> SYSGPIVVDPVTRIEGHLRIEVEVENGKVKNAYSSSTLFRGLEIILKGRDPRDAQHFTQRTCGVCTYTHALASTRCVDNAVGVHIPKNATYIRNLVLGAQYLHDHIVHFYHLHALDFVDVTAALKADPAKAAKVASSISPRKTTAADLKAVQDKLKTFVESGQLGPFTNAYFLGGHPAYYLDPETNLIATAHYLEALRLQVKAARAMAVFGAKNPHTQFTVVGGVTCYDALTPQRIAEFEALWKETKAFVDEVYIPDLLVVAAAYKDWTQYGGTDNFITFGEFPKDEYDLNSRFFKPGVVFKRDFKNIKPFDKMQIEEHVRHSWYEGAEARHPWKGQTQPKYTDLHGDDRYSWMKAPRYMGEPMETGPLAQVLIAYSQGHPKVKAVTDAVLAKLGVGPEALFSTLGRTAARGIETAVIAEYVGVMLQEYKDNIAKGDNVICAPWEMPKQAEGVGFVNAPRGGLSHWIRI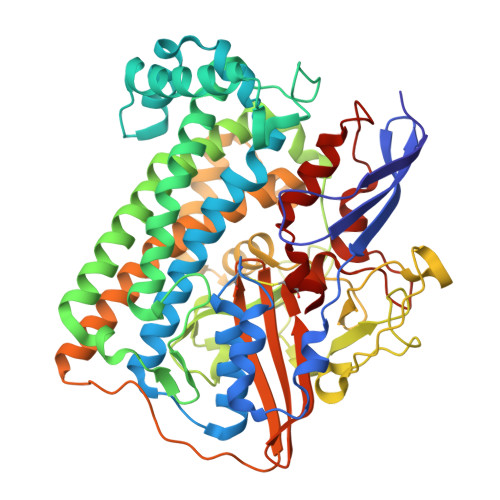EDGKIGNFQLVVPSTWTLGPRCDKNKLSPVEASLIGTPVADAKRPVEILRTVHSFDPCIACGVH> MAKQYDSVECPFCDEVSKYEKLAKIGQGTFGEVFKARHRKTGQKVALKKVLMENEKEGFPITALREIKILQLLKHENVVNLIEICRTKASPYNRCKGSIYLVFDFCEHDLAGLLSNVLVKFTLSEIKRVMQMLLNGLYYIHRNKILHRDMKAANVLITRDGVLKLADFGLARAFSLAKNSQPNRYTNRVVTLWYRPPELLLGERDYGPPIDLWGAGCIMAEMWTRSPIMQGNTEQHQL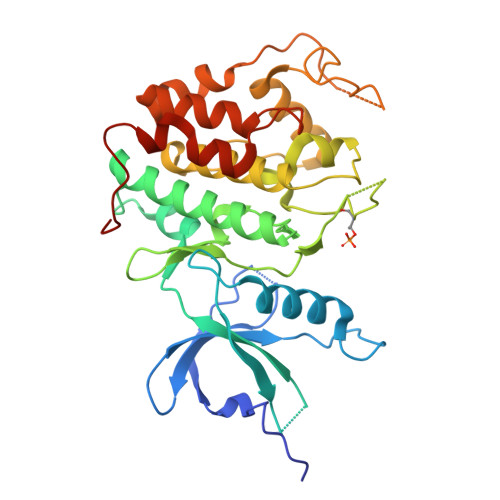ALISQLCGSITPEVWPNVDNYELYEKLELVKGQKRKVKDRLKAYVRDPYALDLIDKLLVLDPAQRIDSDDALNHDFFWSDPMPSDLKGMLST(3R)-3-(aminomethyl)-9-methoxy-1,2,3,4-tetrahydro-5H-[1]benzothieno[3,2-e][1,4]diazepin-5-one | 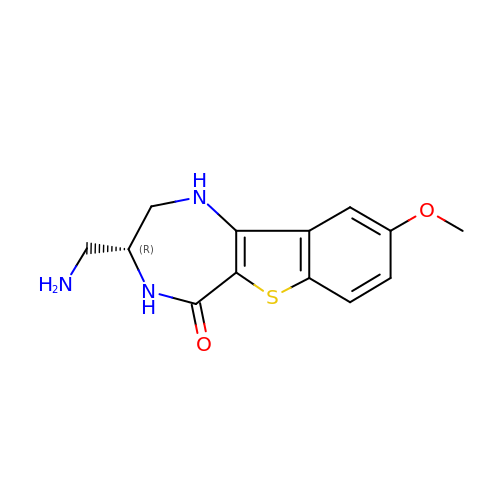C13 H15 N3 O2 S | TXYKBKYDFZQOCB-SSDOTTSWSA-N(2-methoxy-4-methoxycarbonyl-phenyl) 5-nitrofuran-2-carboxylate | C14 H11 N O8 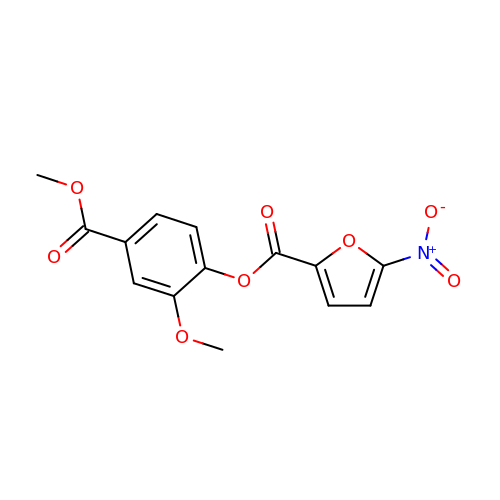| GPPPJBXPBOWUNP-UHFFFAOYSA-N>[2x]MGHHHHHHENLYFQGSMHNDKDLSTWQTFRRLWPTIAPFKAGLIVAGVALILNAASDTFMLSLLKPLLDDGFGKTDRSVLVWMPLVVIGLMILRGITSYVSSYCISWVSGKVVMTMRRRLFGHMMGMPVSFFDK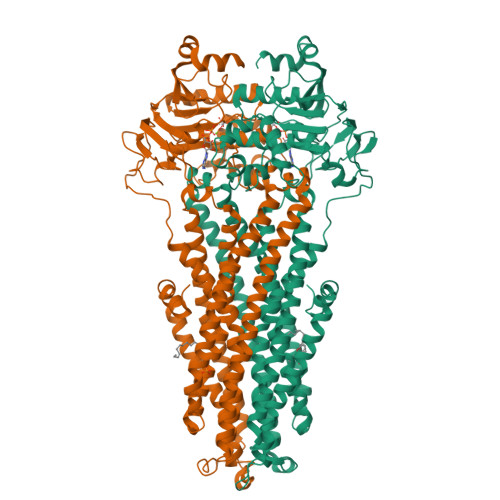QSTGTLLSRITYDSEQVASSSSGALITVVREGASIIGLFIMMFYYSWQLSIILIVLAPIVSIAIRVVSKRFRNISKNMQNTMGQVTTSAEQMLKGHKEVLIFGGQEVETKRFDKVSNRMRLQGMKMVSASSISDPIIQLIASLALAFVLYAASFPSVMDSLTAGTITVVFSSMIALMRPLKSLTNVNAQFQRGMAACQTLFTILDSEQEKDEGKRVIERATGDVEFRNVTFTYPGRDVPALRNINLKIPAGKTVALVGRSGSGKSTIASLITRFYDIDEGEILMDGHDLREYTLASLRNQVALVSQNVHLFNDTVANNIAYARTEQYSREQIEEAARMAYAMDFINKMDNGLDTVIGENGVLLSGGQRQRIAIARALLRDSPILILDEATSALDTESERAIQAALDELQKNRTSLVIAHRLSTIEKADEIVVVEDGVIVERGTHNDLLEHRGVYAQLHKMQFGQ> MRVLVTGGAGFIGSHIVEDLLARGLEVAVLDNLATGKRENVPKGVPFFRVDLRDKEGVERAFREFRPTHVSHQAAQASVKVSV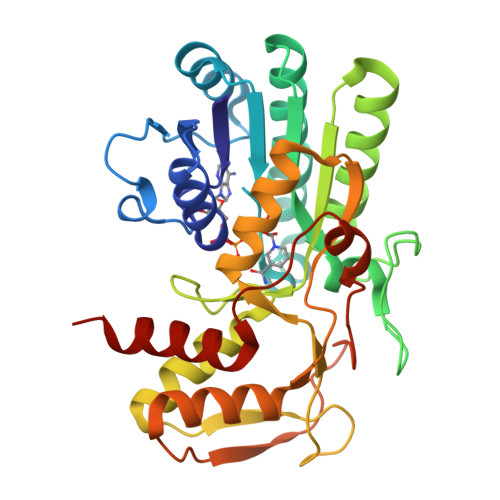EDPVLDFEVNLLGGLNLLEACRQYGVEKLVFASTGGAIYGEVPEGERAEETWPPRPKSPYAASKAAFEHYLSVYGQSYGLKWVSLRYGNVYGPRQDPHGEAGVVAIFAERVLKGLPVTLYARKTPGDEGCVRDYVYVGDVAEAHALALFSLEGIYNVGTGEGHTTREVLMAVAEAAGKAPEVQPAPPRPGDLERSVLSPLKLMAHGWRPKVGFQEGIRLTVDHFRGAV>[4x]MEDPEDPFTRYALAQEHLKHDNASRALALFEELVETDPDYVGTYYHLGKLYERLDR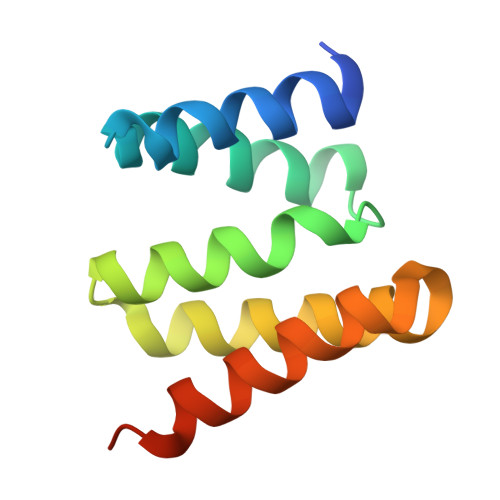TDDAIDTYAQGIEVAREEGTQKDLSELQDAKLKAEGLEHHHHHH>MQYEKVKPPENGEKIRYENGKLIVPDNPIIPYFEGDGIGKDVVPAAIRVLDAAADKIGKEVVWFQVYAGEDAYKLYGNYLPDDTLNAIKEFRVALKGPLTTPVGGGYRSLNVTIRQVLDLYANVRPVYYLKGVPSPIKHPEKVNFVIFRENTEDVYAGIEWPRGSEEALKLIRFLKNEFGVTIREDSGIGIKPISEFATKRLVRMAIRYAIENNRKSVTLVHKGNIMKYTEGAFRDWGYEVAKQEFGEYCITEDELWDKYGGKQPEGKIVVKDRIADNMFQQILTRTDEYDVIALPNLNGDYLSDAAAALIGGLGIAPGSNIGDGIGVFEPVHGSAPKYAGQ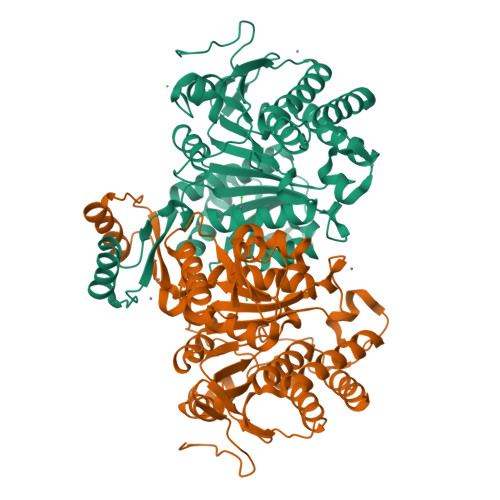NKVNPTAEILTGALMFEYIGWKDASEMIKKAVEMTISSGIVTYDIHRHMGGTKVGTREFAEAVVENLQSL[2x]> SGDYRVQNTSLEAIVQNASSDNQGIQLSAVQAARKLLSSDRNPPIDDLIKSGILPILVHCLERDDNPSLQFEAAWALTNIASGTSEQTQAVVQSNAVPLFLRLLHSPHQNVCEQAVWALGNIIGDGPQCRDYVISLGVVKPLLSFISPSIPITFLRNVTWVMVNLCRHKDPPPPMETIQEILPALCVLIHHTDVNILVDTVWALSYLTDAGNEQIQMVIDSGIVPHLVPLLSHQEVKVQTAALRAVGNIVTGTDEQTQVVLNCDALSHFPALLTHPKEKINKEAVWFLSNITAGNQQQVQAVIDANLVPMIIHLLDKGDFGTQKEAAWAISNLTISGRKDQVAYLIQQNVIPPFCNLLTVKDAQVVQVVLD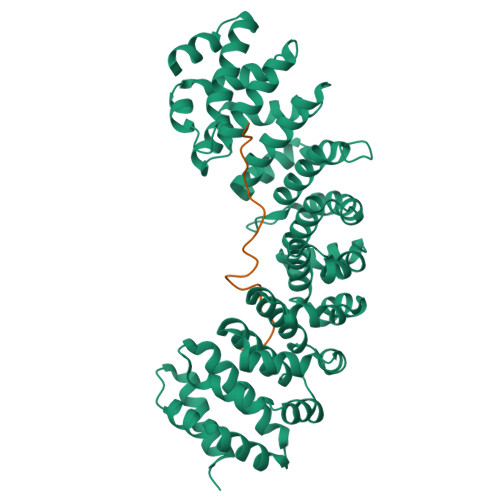GLSNILKMAEDEAETIGNLIEECGGLEKIEQLQNHENEDIYKLAYEIIDQFFSSDDIDEDPSLVPEAIQGGTFGFNSSANVPTEGFQF;> SRNIHLLGRKTCLGRRVVQPGMFEDHPPTKKARVSMRRMSN>[6x]MTVTDIILIHGALNRGACYDAVVPLLEARGYRVHAPDLTGHTPGDGGHLSVVDMEHYTRPVADILARAEGQSILLGHSLGGASISWLAQH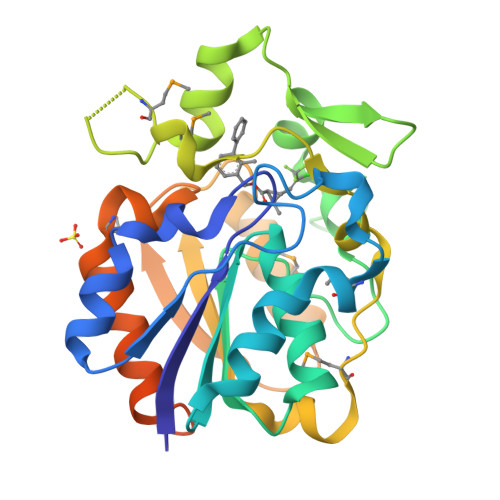HPDKVAGLIYLTAVLTAPGVTPETFVLPGEPNRGTPHALDLIQPVDEGRGLQADFSRLERLREVFMGDYPGEGMPPAEHFIQTQSTVPFGTPNPMEGRALEIPRLYIEALDDVVLPIAVQRQMQKEFPGPVAVVSLPASHAPYYSMPERLAEAIADFADAPAEYRQTATKAGPDRPAGADGGRADRADLPLEHHHHHH Protein phosphatase 2A (PP2A) is a major Ser/Thr protein phosphatase that together with Protein phosphatase 1 accounts for more than 90% of all dephosphorylation events in any given tissue or eukaryotic cell. Each holoenzyme consists of a common core formed by the scaffolding (A) and the catalytic (C) subunit (two isoforms each) and associates with a variable regulatory B-subunit into a heterotrimeric complex. Within the holoenzyme, the regulatory B-subunits control the function of PP2A by mediating substrate specificity and modulating the catalytic activity. Unique for this B-subunit family is the conservation of two EF-hand calcium binding motifs, which are important for the function of the protein.

As an alternative approach, we identified a chymotrypsin resistant core of the PR70 subunit (residues 130–483) using limited proteolysis together with mass spectrometry. The structure of the PR70 core fragment (residues 130–483) was solved by selenomethionine single anomalous dispersion (SAD) phasing and refined at 2 Å resolution yielding a final Rfree of 19.3% (Rwork = 16.2%). However, we find that the structure can be more accurately described as a tandem of two calcineurin B-like domains, which we have named CBLD1 and CBLD2, connected by a 12-residue linker (residues 301–312). Calcineurin B-like domains contain four EF-hands, which are arranged into two so called EF-lobes, i.e. pairs of tightly interacting EF-hands. In agreement with previous observations, only two of the EF hands of PR70 are loaded with calcium. These EF hands correspond to EF5 and EF7 in the present structure, but have in the previous literature been referred to as EF1 and EF2 respectively. On the other hand, EF5 is distinctly non-canonical: it lacks the two conserved glycine residues, and position twelve is occupied by an aspartate. However, in EF5, the aspartate does not interact directly with the Ca2+ ion, but forms a single indirect interaction mediated by a water molecule instead. As a result of this unusual arrangement, the chelated Ca2+ ion is coordinated by only six atoms in an octahedral pattern, with two of them being water molecules. The structure of PR70 in the heterotrimer shows small but significant structural differences as compared with free PR70, supporting a degree of induced fit upon binding.

> SMFPRGRPQDSVNVDAVISKIESTFARFPHERATMDDMGLVAKACGCPLYWKGPLFYGAGGERTGSVSVHKFVAMWRKILQNCHDDAAKFVHLLMSPGCNYLVQEDFVPFLQDVVNTHPGLSFLKEASEFHSRYITTVIQRIFYAVNRSWSGRITCAELRRSSFLQNVALLEEEADINQLTEFFSYEHFYVIYCKFWELDTDHDLLIDADDLARHNDHALSTKMIDRIFSGAVTRGRKVQKEGKISYADFVWFLISEEDKKTPTSIEYWFRCMDLDGDGALSMFELEYFYEEQCRRLDSMAIEALPFQDCLCQMLDLVKPRTEGKITLQDLKRCKLANVFFDTFFNIEKYLDHEQK The type VI secretion systems (T6SSs) of Gram-negative bacteria inject various toxic effectors into the periplasmic or cytoplasmic space of the target cells and induce cell lysis of enemy cells. The various T6SS-related amidase effector proteins (Taes) are classified into four families (Tae1, Tae2, Tae3 and Tae4) based on their cleavage specificities. Tai1, Tai2, Tai3 and Tai4 neutralize the endogenous toxic effectors Tae1, Tae2, Tae3 and Tae4, respectively. To gain insight into the Tae4 family proteins, we determined the crystal structures of Tai4 and of the Tae4–Tai4 complex from Agrobacterium tumefaciens at 1.55 and 1.9 Å resolution, respectively.

The crystal structure of AtTai4 was determined at 1.55 Å resolution. The α2 helix (residues 52–74) contributes to dimer formation in the asymmetric unit, which is consistent with the size-exclusion chromatography results indicating that AtTai4 exists as a dimer in solution. Superimposition of AtTai4 alone and AtTai4 bound to AtTae4 resulted in a root-mean-square deviation (r.m.s.d.) value of 0.8 Å, indicating that no structural changes occur upon complex formation. AtTai4 shares 32.3% amino-acid sequence identity with SmTai4.

>GPGHMAERTWIFSGAELKQAIEGKLAPDVSDPEMRRLVSVAKSSAYIAGVADLTSGSDWCGAGAVAPHELTDRIYTYLGDMPAEKLDEQAATLVREALKVSFPCEQKSN[2x]>EIVKTKRFAIKPMSEEEAVLEMELLGHNFFVFQNGDSNEVNVVYKR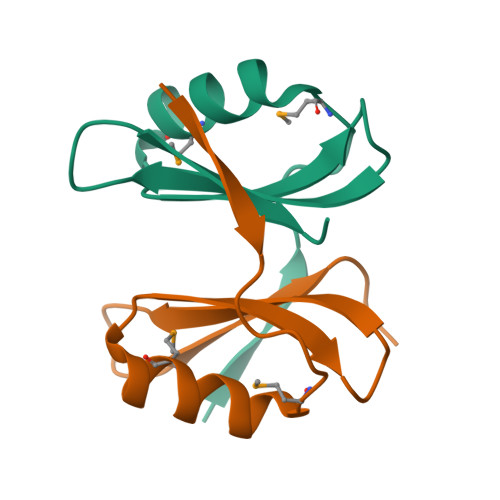KDGNYGLIEPELEHHHHHH[2x]Like all Apicomplexa (the phylum to which Plasmodium belong), malaria parasites move using a substrate-dependent mechanism called gliding motility, a sophisticated substrate-dependent form of cell movement based on a macromolecular complex called the glideosome. At the glideosome core is the single-headed class XIV myosin A (PfMyoA), and short and oriented filaments of a divergent actin (PfAct1). PfMyoA is a tailless myosin consisting only of a motor domain and light chain binding domain. By solving three structural states of the PfMyoA motor domain, corresponding to three states of the motor cycle, we show how the unique class XIV N-terminal heavy chain extension and its interactions with other structural elements define motor function.

Four molecules are present in the asymmetric unit of crystal type 1, one of the motor domain is in the Rigor-like state and three molecules adopt the Post-rigor (PR) state. Second, the interaction between the Relay and the SH1-helix is mainly hydrophobic both in the PPS state and in the Rigor-like state, with the exception of an electrostatic bond between the RelayQ494 and the fulcrum SH2-SH1S691 that is present in the two states. Third, the PfMyoA Rigor-like state is stabilized by atypical interactions of WedgeI587 with Switch-2F473, Switch-2V475, SH2-helixH688 and SH2-SH1S691 (red circle in Fig. 4b). Additional interactions with the N-term extension further stabilize the Rigor-like state, including a strong salt bridge-π interaction between the N-term.extensionGlu6, Switch-1Arg241 and Switch-2Phe476. The electrostatic bond between SEP19 and ConverterK764 stabilizes the Rigor-like conformation while it is unlikely to form in high ADP affinity states. The PfMyoA Rigor-like structure reveals how an interaction of the phosphorylated serine in the N-term extension with the converter is directly involved in the last step of the lever arm swing associated with ADP release. We conclude from the structures that the electrostatic interactions with the N-term extension compensate for the absence of a piston-like movement of the SH1-helix, enabling force production by accelerating the transitions of the powerstroke.

>MAVTNEEIKTASKIVRRVSNVEAFDKSGSVFKGYQIWTDISPTIENDPNIMFVKCVVQQGSKKEKLTVVQIDPPGTGTPYDIDPTHAWNCNSQVDPMSFGDIGLLNHTNIPCVLDFLKHRYLKNQIYTTAVPLIVAINPYKDLGNTTNEWIRRYRDTADHTKLPPHVFTCAREALSNLHGVNKSQTIIVSGESGAGKTEATKQIMRYFASSKSGNMDLRIQTAIMAANPVLEAFGNAKTIRNNNSSRFGRFMQLVISHEGGIRYGSVVAFLLEKSRIITQDDNERSYHIFYQFLKGANSTMKSKFGLKGVTEYKLLNPNSTEVSGVDDVKDFEEVIESLKNMELSESDIEVIFSIVAGILTLGNVRLIEKQEAGLSDAAAIMDEDMGVFNKACELMYLDPELIKREILIKVTVAGGTKIEGRWNKNDAEVLKSSLCKAMYEKLFLWIIRHLNSRIEPEGGFKTFMGMLDIFGFEVFKNNSLEQLFINITNEMLQKNFVDIVFERESKLYKDEGISTAELKYTSNKEVINVLCEKGKSVLSYLEDQCLAPGGTDEKFVSSCATNLKENNKFTPAKVASNKNFIIQHTIGPIQYCAESFLLKNKDVLRGDLVEVIKDSPNPIVQQLFEGQVIEKGKIAKGSLIGSQFLNQLTSLMNLINSTEPHFIRCIKPNENKKPLEWCEPKILIQLHALSILEALVLRQLGYSYRRTFEEFLYQYKFVDIAAAEDSSVENQNKCVNILKLSGLSESMYKIGKSMVFLKQEGAKILTK[4x]(2~{R},3~{S},4~{S})-2,3,4,6-tetrakis(oxidanyl)hexane-1-sulfonic acid | C6 H14 O7 S | 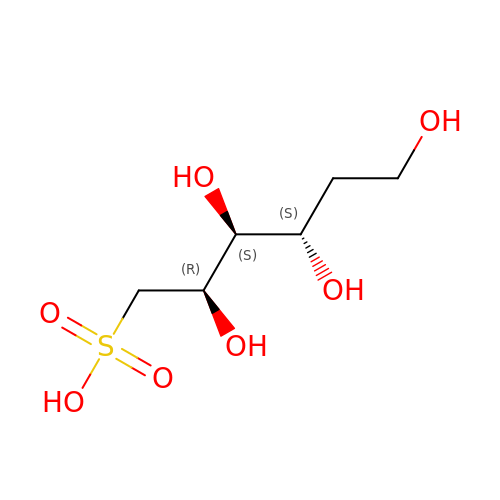CASIPAVAJJTHFL-ZLUOBGJFSA-N>[2x]GRKPIKTLLITGQNNHNWQVSHVVLKQILENSGRFDVDFVISPEQGKDMSGFVLDFSPYQLVVLDYNGDSWPEETNRRFLEYVQNGGGVVIYHAADNAFSKWPEFNRICALGGWEGRNENSGPYVYWKDGKLVKDSSAGPGGSHGRQHEYVLNGRDKVHPVVKGLPLKWRHAKDELYDRMRGPGNIRDILYTAYSDKETNGSGREEPLVFTVDYGN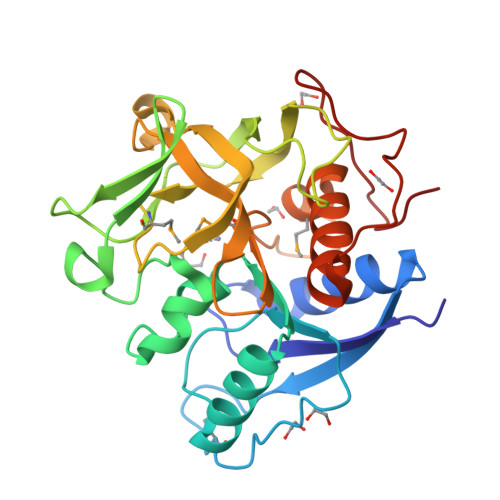ARIFHTMLGHAGATTEDNIAMQCTGFQVLLLRGAEWAATGKVTQKVPKDFPTETTCSYRKDYKEN>GKDEYPLHMAAANDDIQLIKHILSQKTLIDARDETGSTALMVATRANNIHAAHMLIEAGADVNAKDNIQDSPYLYAGAQGYLKILRMTLMHGADLKSTNRYGGTALIPAAERGHVETVRTLIAAGVNVNHVNNLGWTALLEAIILGNGKSNYQQIVALLLKAGANPNLADKDGITPLQHARTRGYREIE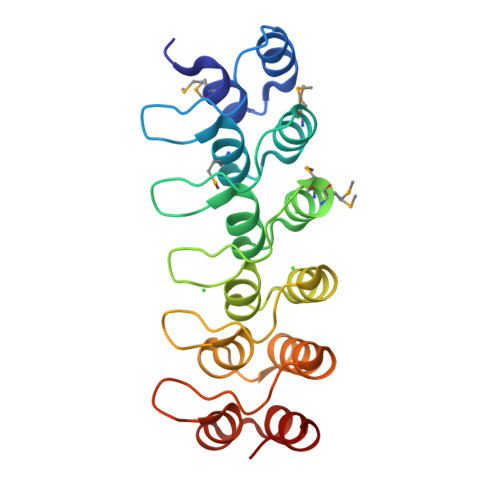KLLLVAGAK[2x]> SPNVE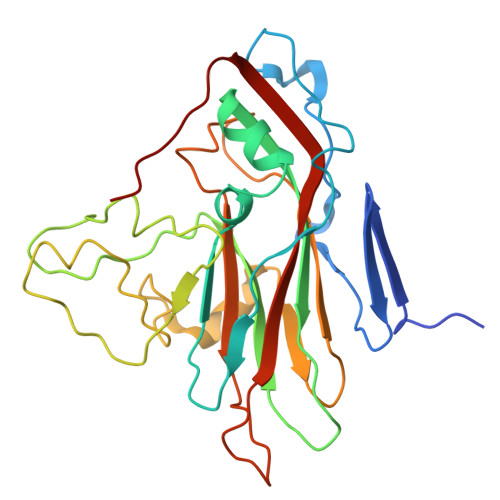ACGYSDRVRQITLGNSTITTQEAANAVVAYGEWPSYLDDKEANPIDAPTEPDVSSNRFYTLDSVQWKSTSRGWWWKLPDALKDMGMFGQNMYYHYLGRSGYTVHVQCNASKFHQGALGVFAIPEYVMACNTEAKTSYVSYVNANPGEKGGVFDNAYNPSAEASEGRKFAALDYLLGCGVLAGNAFVYPHQIINLRTNNSATLVLPYVNSLAIDCMAKHNNWGLVILPLCKLDYAPNSSTEIPITVTIAPMFTEFNGLRNITVPATQ2-(2-CHLORO-4-FLUOROPHENOXY)-2-METHYL-N-[(1R,2S,3S,5S,7S)-5-(METHYLSULFONYL)-2-ADAMANTYL]PROPANAMIDE 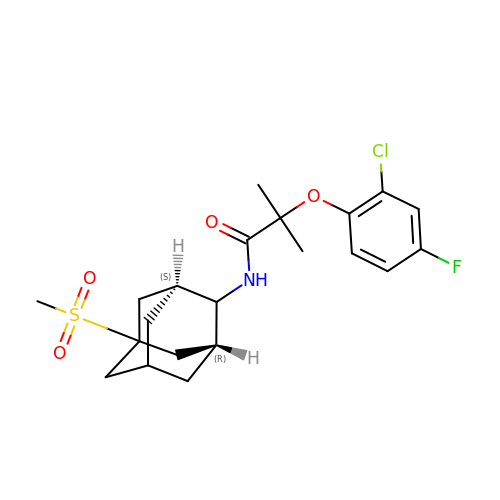| C21 H27 Cl F N O4 S | ULLPKOZNMAWTIP-JGSHYQHOSA-N> MANNDAVLKRLEQKGAEADQIIEYLKQQVSLLKEKAILQATLREEKKLRVENAKLKKEIEELKQELIQAEIQNGVKQIPFPSGTPLHANSMVSENVIQSTAVTTVSSGTKEQIKGGTGDEKKAKEKIEKKGEKKEKKQQSIAGSADSKPIDVSRLDLRIGCIITARKHPDA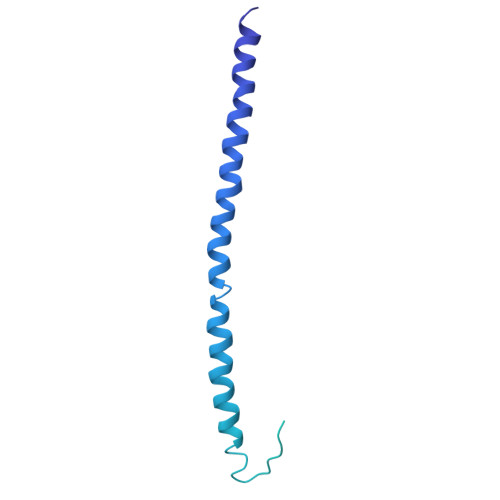DSLYVEEVDVGEIAPRTVVSGLVNHVPLEQMQNRMVILLCNLKPAKMRGVLSQAMVMCASSPEKIEILAPPNGSVPGDRITFDAFPGEPDKELNPKKKIWEQIQPDLHTNDECVATYKGVPFEVKGKGVCRAQTMSNSGIK PXR is a nuclear receptor that can be activated by diverse compounds to elevate metabolism, negatively impacting drug efficacy and safety. As a xenobiotic sensor, PXR is activated by structurally diverse compounds and plays a major role in drug metabolism and drug-drug interactions by regulating transcription of genes encoding drug metabolizing enzymes, drug conjugating enzymes, and drug transporters. Here, we report structurally related PXR-selective agonists and antagonists and their corresponding co-crystal structures to describe mechanisms of antagonism and selectivity. Structural and computational approaches show that antagonists induce PXR conformational changes incompatible with transcriptional coactivator recruitment.

To explore the ligand-mutant interactions and exclude the possibility that a different ligand orientation causes the switch from antagonist to agonist, we obtained crystal structures of PXRL428V LBD apo and bound to the antagonist SJPYT-331. L428V was chosen because (1) it is potently activated by the three ligands, (2) it is a conservative mutation in which the WT residue (Leu) is biochemically similar to the mutated residue (Val), and (3) L428 shifts away from SRC-1 in the antagonist-bound WT PXR LBD structures. The mutation did not alter the overall protein fold, including the position of α12, as compared to WT PXR LBD. The L428V mutation results in increased hydrophobicity, reduced amino acid sidechain size, and reduced rotameric freedom. Accordingly, the M425-V428-F429 contact surface was slightly compacted compared to the M425-L428-F429 surface. The residues M425, L428, and F429 form a hydrophobic “hot spot” that contacts agonists through moieties such as the 4-methoxy group, and mutations may change the nature of the hot spot due to a combination of factors, including hydrophobicity, orientation, and size.

>[2x]HHHHHHGSERTGTQPLGVQGLTEEQRMMIRELMDAQMKTFDTTFSHFKNFRLPGVLSSGCELPESLQAPSREEAAKWSQVRKDLCSLKVSLQLRGEDGSVWNYKPPADSGGKEIFSLLPHMADMSTYMFKGIISFAKVISYFRDLPIEDQISLLKGAAFELCQLRFNTVFNAETGTWECGRLSYCLEDTAGGFQQLLLEPMLKFHYMLKKLQLHEEEYVLMQAISLFSPDRPGVLQHRVVDQLQEQFAITLKSYIECNRPQPAHRFLFLKIMAMLTELRSINAQHTQRLLRIQDIHPFATPLMQEVFGITGSSGGSGGSSHSSLTERHKILHRLLQEGSPSDITTLSVEPD Sortilin can trigger internalization of ligands from the cell surface via endocytosis and sorts ligands between several intracellular compartments, such as the trans-Golgi network (TGN), endosomes, lysosomes, and the secretory pathway. Sortilin binds and sorts a broad range of ligands, and dysfunction of sortilin has been linked to a wide range of disorders. Previously solved crystal structures of s-sortilin revealed that the Vps10p domain in fact consists of three domains; a ten-bladed β-propeller and two 10CC domains (10CC-a and 10CC-b) that have substantial interactions with the β-propeller. In this study, we detail that sortilin undergoes a conformational change within the three luminal domains and dimerizes while transitioning from neutral to acidic pH.

We determined the structures of the glycosylated luminal segment of mouse sortilin, s-sortilin, from crystals grown at neutral pH (pH 7.5, one crystal form, 2.1 Å maximum resolution) and acidic pH (pH ranging from 5.0 to 6.2, three crystal forms, maximum resolution ranging from 2.3 to 4.0 Å). The structures reveal two distinct conformations, a monomer at neutral pH and a dimer at acidic pH. The eight independent s-sortilin molecules in the three crystal forms grown at acidic pH all form homodimers with an identical interface and highly similar structure. The r.m.s.d. between the s-sortilin chains in the dimers is 0.80 Å for all of the 650 Cα atoms modeled. S-sortilin dimerizes through the top face of the β-propeller, i.e., the large side of the β-propeller disk opposite to the bottom face at which the 10CC domains are located. The predominantly hydrophobic dimer interface is large with a buried surface area of 4882 Å2 and is formed mainly by loops protruding from the blades. β-Propeller blades 1, 4, 6, 7, 8, 9, and 10 are involved in dimer formation. In the s-sortilin dimer the C-termini are in close proximity to each other with 37 Å distance between the two N713 Cα atoms. The s-sortilin dimer structures, crystallized at acidic pH, reveal that dimerization is accompanied by a substantial conformational rearrangement within the ß-propeller and two 10CC domains. Despite three internal disulfide bonds in 10CC-b, the three α-helices that form a small hydrophobic core in the s-sortilin monomer change their conformation into a three-stranded β-sheet in the dimer. In the monomer conformation, the s-sortilin C-terminus is exposed and pointing away from the β-propeller; whereas in the dimer conformation, it is interacting, through conserved hydrophobic interactions, with the rim of the β-propeller at blades 4 and 5.

>GQDRLDAPPPPAPPLLRWAGPVGVSWGLRAAAPGGPVPRAGRWRRGAPAEDQDCGRLPDFIAKLTNNTHQHVFDDLSGSVSLSWVGDSTGVILVLTTFQVPLVIVSFGQSKLYRSEDYGKNFKDITNLINNTFIRTEFGMAIGPENSGKVILTAEVSGGSRGGRVFRSSDFAKNFVQTDLPFHPLTQMMYSPQNSDYLLALSTENGLWVSKNFGEKWEEIHKAVCLAKWGPNNIIFFTTHVNGSCKADLGALELWRTSDLGKTFKTIGVKIYSFGLGGRFLFASVMADKDTTRRIHVSTDQGDTWSMAQLPSVGQEQFYSILAANEDMVFMHVDEPGDTGFGTIFTSDDRGIVYSKSLDRHLYTTTGGETDFTNVTSLRGVYITSTLSEDNSIQSMITFDQGGRWEHLRKPENSKCDATAKNKNECSLHIHASYSISQKLNVPMAPLSEPNAVGIVIAHGSVGDAISVMVPDVYISDDGGYSWAKMLEGPHYYTILDSGGIIVAIEHSNRPINVIKFSTDEGQCWQSYVFTQEPIYFTGLASEPGARSMNISIWGFTESFITRQWVSYTVDFKDILERNCEEDDYTTWLAHSTDPGDYKDGCILGYKEQFLRLRKSSVCQNGRDYVVAKQPSVCPCSLEDFLCDFGYFRPENASECVEQPELKGHELEFCLYGKEEHLTTNGYRKIPGDKCQGGMNPAREVKDLKKKCTSNFLNPTKQNSKSNAAAHHHHHH[4x]> MARENEMDENLEQVSGIIGNLRH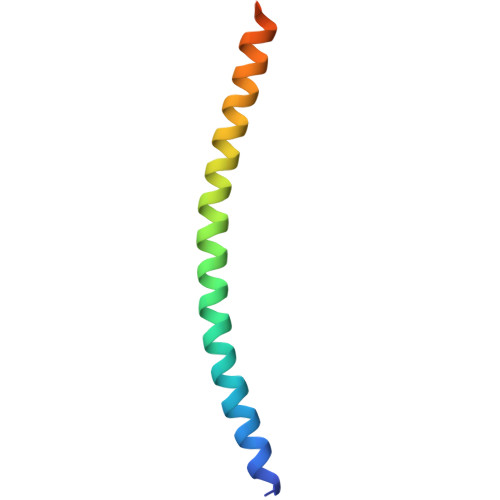MALDMGNEIDTQNRQIDRIMEKADSNKTRIDEANQRATKMLG>HMSQSNRELVVDFLSYKLSQKGYSWSQMAAVKQALREAGDEFELRYRRAFSDLTSQLHITPGTAYQSFEQVVNELFRDGVNWGRIVAFFSFGGALCVESVDKEMQVLVSRIAAWMATYLNDHLEPWIQENGGWDTFVELYGN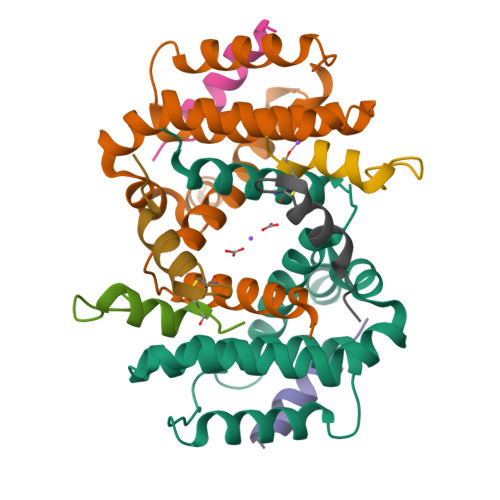NAAAESRKGQE[2x];>DEMFSDIYKIREIADGLCLEV[6x]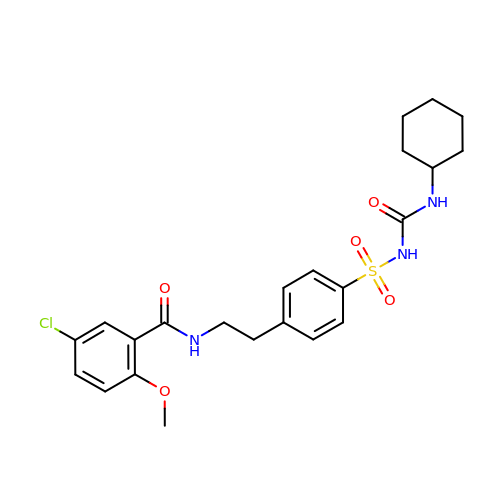5-chloro-N-(2-{4-[(cyclohexylcarbamoyl)sulfamoyl]phenyl}ethyl)-2-methoxybenzamide | C23 H28 Cl N3 O5 S | ZNNLBTZKUZBEKO-UHFFFAOYSA-N One intriguing example is the African swine fever virus, which stands as the sole mammalian-infecting virus encoding a type II topoisomerase. The ORF P1192R encodes a functional Topo II (pP1192R) which is highly conserved across diverse ASFV isolates. Prior extensive structural and biochemical studies have elucidated key aspects of Topo II catalytic mechanisms. These structures have unveiled the inherent architecture of Topo II, which is characterized by two principal heart-shaped functional domains: the ATPase domain, responsible for ATP hydrolysis to fuel the molecular machinery, and the central domain, which interacts with the DNA duplex and contains a catalytic tyrosine residue that cleaves the DNA duplex. As a result, Topo II not only relaxes DNA supercoiling but also disentangles knots and catenates potentially detrimental to cellular function if left unresolved.

The apo pP1192R (full-length and the central domain) were plunged-frozen on an amorphous alloy film (R1.2/1.3, Au, 300 mesh) at the concentration of 0.8 mg/ml. As indicated by our structural analyses, without DNA binding, the apo pP1192R undergoes dynamic conformational changes. Notably, three distinct apo conformations exist: pP1192RClose, pP1192RCoil-open and pP1192RWHD-open. A comparative analysis of the three apo central domain structures (pP1192RClose, pP1192RCoil-open and pP1192RWHD-open) reveals that notable conformational shifts are evident within these structures. Compared with pP1192RCoil-open and pP1192RClose, pP1192RWHD-open exhibits an apparent separation of ~26 Å between the WHD subdomains. Compared with pP1192RCD-DNA, two catalytic Y800 of pP1192RWHD-open also rotate by ~40° and the distance stretches to 32.6 Å. The diverse positions of Y800 across these conformations serve as indicators of the distinct functional states adopted by pP1192R.

>EFATMEAFEISDFKEHAKKKSMWAGALNKVTISGLMGVFTEDEDLMALPIHRDHCPALLKIFDEIIVNATDHERACHNKTKKVTYIKISFDKGVFSCENDGPGIPIAKHEQASLIAKRDVYVPEVASCHFLAGTNINKAKDCIKGGTNGVGLKLAMVHSQWAILTTADGAQKYVQHINQRLDIIEPPTITPSREMFTRIELMPVYQELGYAEPLSETEQADLSAWIYLRACQCAAYVGKGTTIYYNDKPCRTGSVMALAKMYTLLSAPNSTIHTATIKADAKPYSLHPLQVAAVVSPKFKKFEHVSVINGVNCVKGEHVTFLKKTINEMVVKKFQQTIKDKNRKTTLRDSCSNIFIVIVGSIPGIEWTGQRKDELSIAENVFKTHYSIPSSFLTSMTKSIVDILLQSISKKDNHKQVDVDKYTRARNAGGKRAQDCMLLAAEGDSALSLLRTGLTLGKSNPSGPSFDFCGMISLGGVIMNACKKVTNITTDSGETIMVRNEQLTNNKVLQGIVQVLGLDFNCHYKTQEERAKLRYGCIVACVDQDLDGCGKILGLLLAYFHLFWPQLIIHGFVKRLLTPLIRVYEKGKTMPVEFYYEQEFDAWAKKQTSLANHTVKYYKGLAAHDTHEVKSMFKHFDNMVYTFTLDDSAKELFHIYFGGESELRKRELCTGVVPLTETQTQSIHSVRRIPCSLHLQVDTKAYKLDAIERQIPNFLDGMTRARRKILAGGVKCFASNNRERKVFQFGGYVADHMFYHHGDMSLNTSIIKAAQYYPGSSHLYPVFIGIGSFGSRHLGGKDAGSPRYISVQLASEFIKTMFPAEDSWLLPYVFEDGQRAEPEYYVPVLPLAIMEYGANPSEGWKYTTWARQLEDILALVRAYVDKDNPKHELLHYAIKHKITILPLRPSNYNFKGHLKRFGQYYYSYGTYVISEQRNIITITELPLRVPTVAYIESIKKSSNRMTFIEEIIDYSSSETIEILVKLKPNSLNRIVEEFKETEEQDSIENFLRLRNCLHSHLNFVKPKGGIIEFNTYYEILYAWLPYRRELYQKRLMREHAVLKLRIIMETAIVRYINESAELNLSHYEDEKEASRILSEHGFPPLNHTLIISPEFASIEELNQKALQGCYTYILSLQARELLIAAKTRRVEKIKKMQARLDKVEQLLQESPFPGASVWLEEIDAVEKAIIKGRNTQWKFHENLYFQGHHHHHHHH[2x]> TVPDNLKKQLAVSVRNIQWSYGIFWSVSASQPGVLEWGDGYYNGDIKTRKTIQAAEVKIDQLGLERSEQLRELYESLSLAESSASGSSQVTRRASAAALSPEDLTDTEWYYLVCMSFVFNIGEGIPGGALSNGEPIWLCNAETADSKVFTRSLLAKSASLQTVVCFPFLGGVLEIGTTEHIKED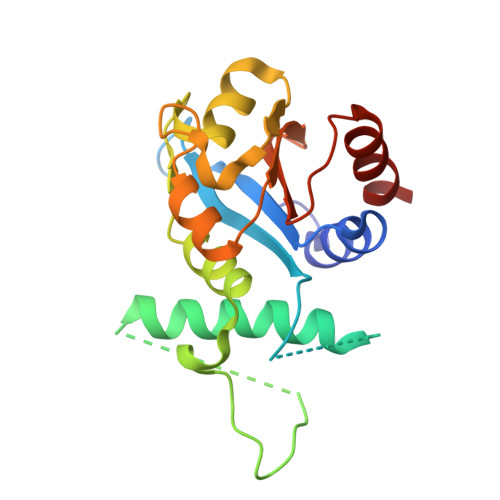MNVIQSVKTLFLEA> GIDPFTAILSEKPNVKWEDVAGLEGAKEALKEAVILPVKFPHLFKGNRKPTSGILLYGPPGTGKSYLAKAVATEANSTFFSVSSSDLVSKWMGESEKLVKQLFAMARENKPSIIFIDQVDALTGTRGEGESEASRRIKTELLVQMNGVGNDSQGVLVLGATNIPWQLDSAIRRRFERRIYIPLPDLAARTTMFEINVGDTPCVLTKEDYRTLGAMTEGYSGSDIAVVVKDALMQPIRKIQSATHFKDVSTEDDETRKLTPCSPGDDGAIEMSWTDIEADELKEPDLTIKDFLKAIKSTRPTVNEDDLLKQ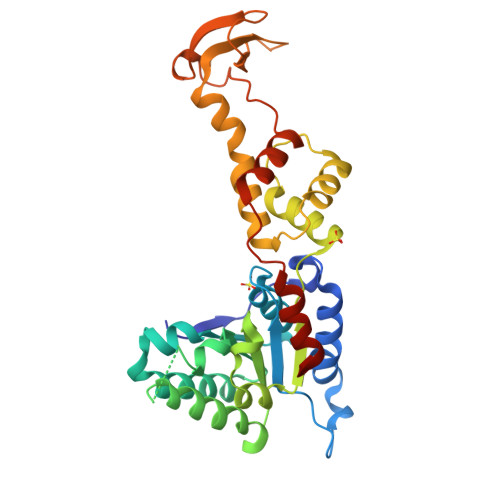EQFTRDFGQEGN>MAKNTITKTLKLRIVRPYNSAEVEKIVADEKNNREKIALEKNKDKVKEACSKHLKVAAYCTTQVERNACLFCKARKLDDKFYQKLRGQFPDAVFWQEISEIFRQLQKQAAEIYNQSLIELYYEIFIKGKGIANASSVEHYLSDVCYTRAAELFKNAAIASGLRSKIKSNFRLKELKNMKSGLPTTKSDNFPIPLVKQKGGQYTGFEISNHNSDFIIKIPFGRWQVKKEIDKYRPWEKFDFEQVQKSPKPISLLLSTQRRKRNKGWSKDEGTEAEIKKVMNGDYQTSYIEVKRGSKICEKSAWMLNLSIDVPKIDKGVDPSIIGGIDVGVKSPLVCAINNAFSRYSISDNDLFHFNKKMFARRRILLKKNRHKRAGHGAKNKLKPITILT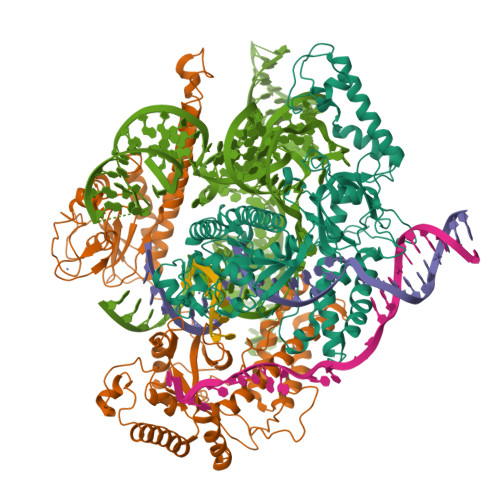EKSERFRKKLIERWACEIADFFIKNKVGTVQMENLESMKRKEDSYFNIRLRGFWPYAEMQNKIEFKLKQYGIEIRKVAPNNTSKTCSKCGHLNNYFNFEYRKKNKFPHFKCEKCNFKENADYNAALNISNPKLKSTKEEP[2x]>VCTEPLGLKDNTIPNKQITASSYYKTWGLSAFSWFPYYARLDNQGKFNAWTAQTNSASEWLQIDLGSQKRVTGIITQGARDFGHIQYVAAYRVAYGDDGVTWTEYKDPGASESKIFPGNMDNNSHKKNIFETPFQARFV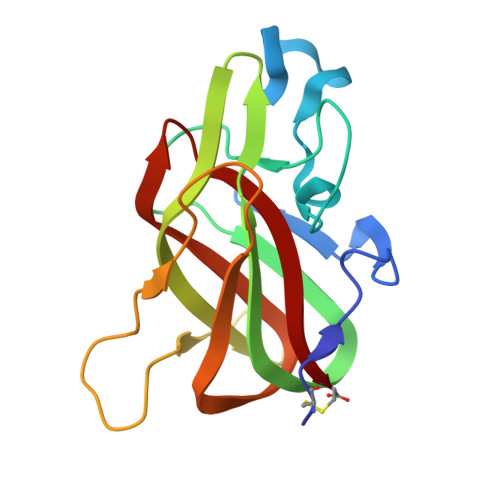RIQPVAWHNRITLRVELLGC[4x]> TDTTLPPDDSLDRIEPVDIEQEMQRSYIDYAMSVIVGRALPEVRDGLKPVHRRVLYAMFDSGFRPDRSHAKSARSVAETMGNYHPHGDASIYDSLVRMAQPWSLRYPLVDGQGNFGSPGNDPPAAMRFTEARLTPLAMEMLREIDEETVDFIPNYDGRVQEPTVLPSRFPNLLANGSGGIAVGMATNIPPHNLRELADAVFWALENHDAD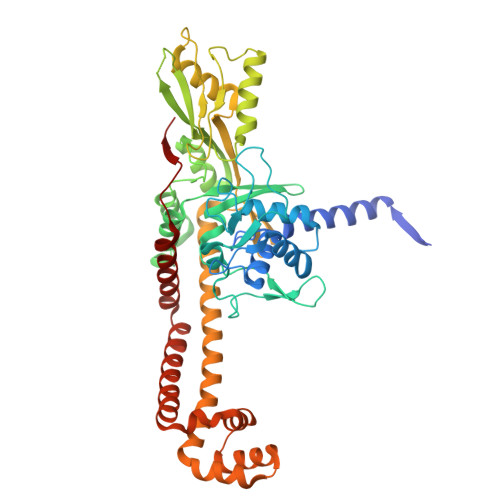EEETLAAVMGRVKGPDFPTAGLIVGSQGTADAYKTGRGSIRMRGVVEVEEDSRGRTSLVITELPYQVNHDNFITSIAEQVRDGKLAGISNIEDQSSDRVGLRIVIEIKRDAVAKVVINNLYKHTQLQTSFGANMLAIVDGVPRTLRLDQLIRYYVDHQLDVIVRRTTYRLRKANERAHILRGLVKALDALDEVIALIRASETVDIARAGLIELLDIDEIQAQAILDMQLRRLAALERQRIIDDLAKIEAEIADLEDILAKPERQRGIVRDELAEIVDRHGDDRRTRIIAA>MSLNSEAKSRIACDIDFDRDGRQAGYARAPLSRNNSGWGTVEIPITVVKNGSGPTVLLTGGVHGDEYEGQIAISDLARRLRPEEVQGRVIMLPAVNMPAIQSDTRLSPVDGRDINRCFPGDPRGTFSQMLAHFLDSVILPMADISVDMHTAGHSYDSTPSTNMHYLADPALRARTLAAAEAFGAPHNVVFGGVDEGSTFTSCVERRGIVSLGTELGGWGRVNIEGVRIGKRGILNVLKHMGVIEGTPETAQRGGAAGTRHMMVREADAYVMAPRTGLFEPTHYVGEEVRTGETAGWIHFVEDV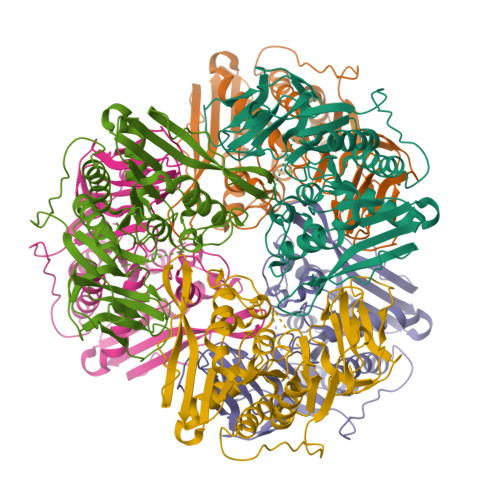DTAPLELLYRRDGIVWFGAGPGRVTRGDAVAVVMEDYNDTWPQEGHHHHHH[6x]>[2x]MRLTILGMTAHDSRPEQAKKLADIDWSTLGFSYIRTDLRYLAHWKDGEWDAGTLTEDNQIHLAEGSTALHYGQQCFEGLKAYRCADGSINLFRPDQNAARMRMSCRRLLMPELSDEQFIDACLQVVRANEHFLPPYGTGGSLYLRPFVIGVGDNIGVRTAPEFIFSVFCVPVGPYFKGGLTPTNFITSDYDRAAPHGTGAAKVGGNYAASLLPGYEAKKRDFADVIY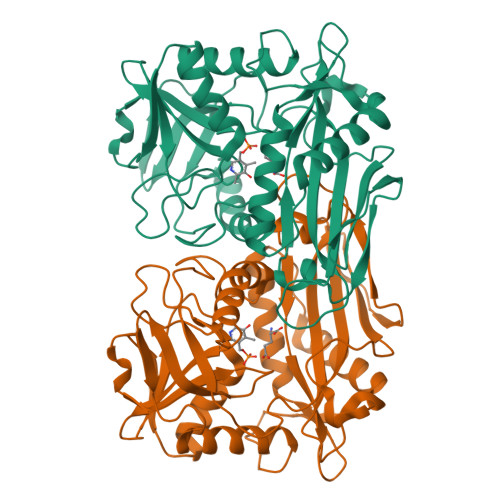LDPATHTTIEEAGAANFFAITQDGQKFVTPQSPSILPSITKYSLLWLAEHRLGLEVEEGDIRIDELGKFSEAGACGTAAVITPIGGIQHGDDFHVFYSESEPGPVTRRLYDELVGIQYGDKEAPEGWIVKV> LIPNISPDSFTVAASTGMLSGKSHEMLYDAETGRKISQLDWKIKNVAILKGDISWDPYSFLTLNARGWTSLAS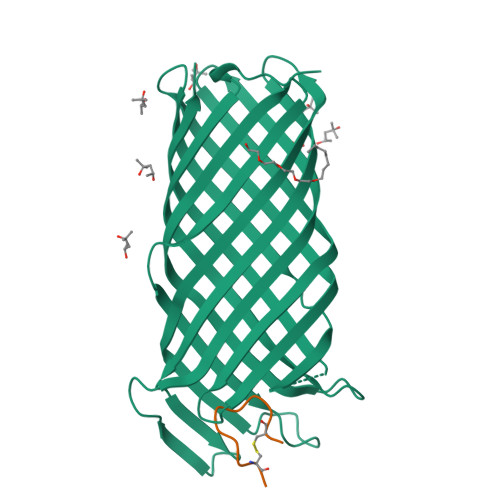GSGNMDNYDWMNENQSEWTDHSSHPATNVNHANEYDLNVKGWLLQDENYKAGITAGYQETRFSWTATGGSYSYNNGAYTGNFPKGVRVIGYNQRFSMPYIGLAGQYRINDFELNALFKFSDWVRAHDNDEHYMRDLTFREKTSGSRYYGTVINAGYYVTPNAKVFAEFTYSKYDEGKGGTQTIDKNSGDSVSIGGDAAGISNKNYTVTAGLQYRFGGGHHHHHH;> KCPGRVVGGCK>[5x]ETTSCEFSVSPSGLAFCDKVVGYGPEAVKGQL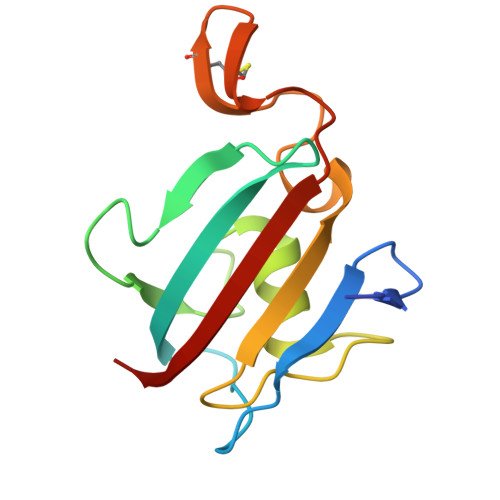IKAHYVGKLENGKVFDSSYNRGKPLTFRIGVGEVIKGWDQGILGSDGIPPMLTGGKRTLRIPPELAYGDRGAGCKGGSCLIPPASVLLFDIEYIGKA> GHMLGFKAERLRVNLRLVINRLKLLEKKKTELAQKARKEIADYLAAGKDERARIRVEHIIREDYLVEAMEILE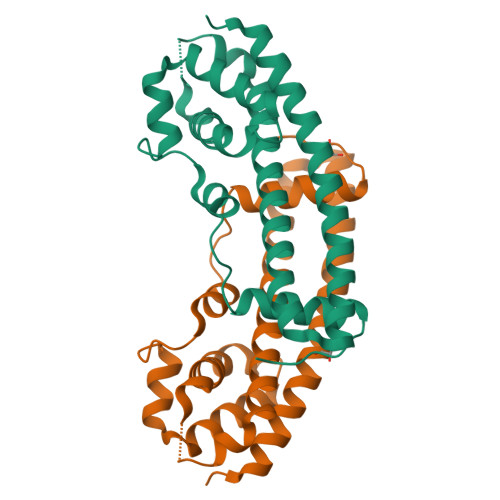LYCDLLLARFGLIQSMKELDSGLAESVSTLIWAAPRLQSEVAELKIVADQLCAKYSKEYGKLCRTNQIGTVNDRLMHKLSVEAPPKILVERYLIEIAKNYNVPYEPDSVVMAEAPP> SLSCRPPMVKLVCPADNLRAEGLECTKTCQ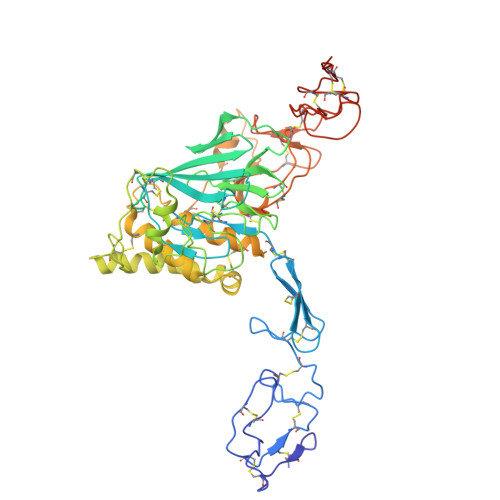NYDLECMSMGCVSGCLCPPGMVRHENRCVALERCPCFHQGKEYAPGETVKIGCNTCVCQDRKWNCTDHVCDATCSTIGMAHYLTFDGLKYLFPGECQYVLVQDYCGSNPGTFRILVGNKGCSHPSVKCKKRVTILVEGGEIELFDGEVNVKRPMKDETHFEVVESGRYIILLLGKALSVVWDRHLSISVVLKQTYQEKVCGLCGNFDGIQNNDLTSSNLQVEEDPVDFGNSWKVSSQCADTRKVPLDSSPATCHNNIMKQTMVDSSCRILTSDVFQDCNKLVDPEPYLDVCIYDTCSCESIGDCACFCDTIAAYAHVCAQHGKVVTWRTATLCPQSCEERNLRENGYECEWRYNSCAPACQVTCQHPEPLACPVQCVEGCHAHCPPGKILDELLQTCVDPEDCPVCEVAGRRFASGKKVTLNPSDPEHCQICHCDVVNLTCEACQEPGGLVVPPHHHHHH The fruit fly Drosophila melanogaster expresses a long-chain fatty acyl-CoA synthetase (ACSL), CG6178, which is 41% identical to Photinus pyralis firefly luciferase (Fluc). Insect ACSLs are promiscuous enzymes, recognizing a variety of fatty acid substrates. However, unlike fireflies and other bioluminescent beetles, nonluminescent insects such as fruit flies do not biosynthesize D-luciferin, which is required for light emission in beetles.6 Moreover, despite its homology to Fluc, CG6178 has been shown to be incapable of adenylating D-luciferin, and does not emit light when treated with d-luciferin and ATP. Nonetheless, further characterization of CG6178 has revealed that the enzyme is a latent luciferase capable of catalyzing light emission, not from d-luciferin, but from synthetic luciferin analogues such as CycLuc2.7,8 Although this latent luciferase activity is relatively weak, it suggests that fatty acyl-CoA synthetases can inform us about how beetle luciferases evolved from their evolutionary antecedents.

Here we report the crystal structure of CG6178, which shares the same overall fold as firefly luciferase, but has a steric protrusion occluding its substrate binding site. The crystal structure of CG6178 was refined to 2.5 Å resolution with a crystallographic R-value of 0.19 and an R-free value of 0.25. 534 out of 544 residues in the CG6178 protein sequence were resolved in the electron density. The first methionine residue, last six residues, and a section from 223–225 were not resolved. The addition of ATP dramatically improved crystallization, but surprisingly, density for ATP is not observed within this structure. Rather, the electron density maps are consistent with an adenylated fatty acid. No fatty acids were explicitly added, but CG6178 is known to accept fatty acid substrates ranging in chain length from C8 to C20.2 The presence of octanoyl-AMP (C8) and an ethylene glycol in the active site is most consistent with the data. Comparing the active sites of CG6178 and Fluc, residues 342–347 of CG6178 create a protrusion that occludes the binding pocket relative to the corresponding sequence in Fluc, especially due to the Leu346 sidechain. We hypothesized that fatty acid substrates can readily traverse this narrow constriction, whereas the relatively bulky d-luciferin cannot, or at least not in a conformation suitable for attack of its carboxylate on ATP during the adenylation step. We mutated the leucine and surrounding residues that comprise this bump and found that mutation of just two residues was sufficient to improve light emission by 20-fold, while also lowering the Km for CycLuc2 by ~7-fold.

> GPLGSMTSKLLPGNIVYGGPVTERQAQDSRSLGQYILDKYKSFGDRTVLVDAVNGVEYSASFMHKSIVRLAYILQKLGVKQNDVVGLSSENSVNFALAMFAGLAVGATVAPLNVTYSDREVDHAINLSKPKIIFASKITIDRVAKVASKNKFVKGIIALSGTSKKFKNIYDLKELMEDEKFKTQPDFTSPAANKDEDVSLIVCSSGTTGLPKGVQLTQMNLLATLDSQIQPTVIPMEEVTLLTVIPWFHAFGCLTLITTACVGARLVYLPKFEEKLFLSAIEKYRVMMAFMVPPLMVFLAKHPIVDKYDLSSLMVLLCGAAPLSRETEDQIKERIGVPFIRQGYGLSESTLSVLVQNDEFCKPGSVGVLKVGIYAKVIDPDTGKLLGANERGELCFKGDGIMKGYIGDTKSTQTAIKDGWLHTGDIGYYDDDFEFFIVDRIKELIKYKGYQVPPAEIEALLLTNDKIKDAAVIGKPDEEAGELPLAFVVKQANVQLTENEVIQFVNDNASPAKRLRGGVIFVDEIPKNPSGKILRRILREMLKKQKSKL>MMVISEKVRKALNDQLNREIYSSYLYLSMATYFDAEGFKGFAHWMKKQAQEELTHAMKFYEYIYRRGGRVELEAIEKPPSNWNGIKDAFEAALKHEEFVTQSIYNILEL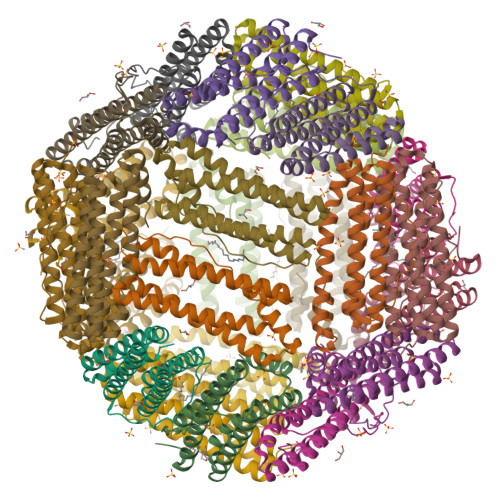ASEEKDHATVSFLKWFVDEQVEEEDQVREILDLLEKANGQMSVIFQLDRYLGQRE[8x]> 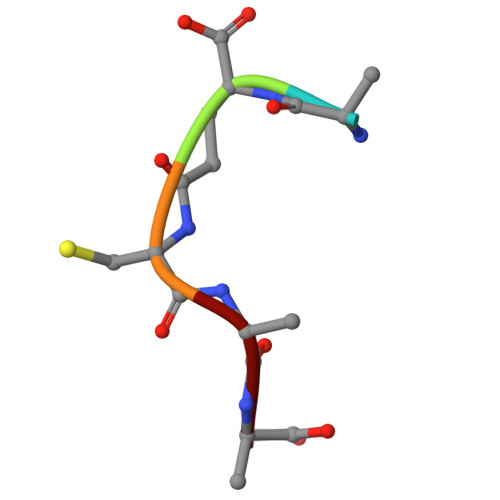AECAA> MGKIIGIDLGTTNSCVAIMDGTTPRVLENAEGDRTTPSIIAYTQDGETLVGQPAKRQAVTNPQNTLFAIKRLIGRRFQDEEVQRDVSIMPFKIIAADNGDAW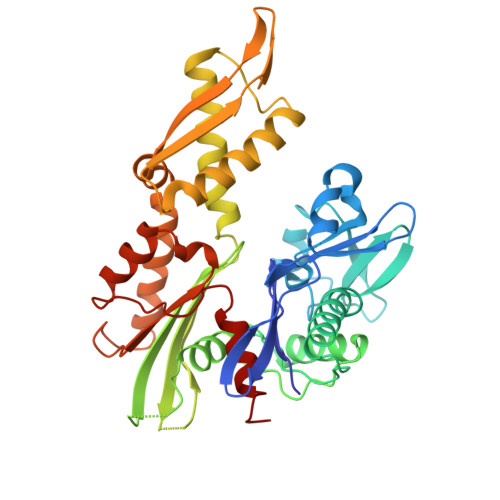VEVKGQKMAPPQISAEVLKKMKKTAEDYLGEPVTEAVITVPAYFNDAQRQATKDAGRIAGLEVKRIINEPTAAALAYGLDKGTGNRTIAVYDLGGGTFDISIIEIDEVDGEKTFEVLATNGDTHLGGEDFDSRLINYLVEEFKKDQGIDLRNDPLAMQRLKEAAEKAKIELSSAQQTDVNLPYITADATGPKHMNIKVTRAKLESLVEDLVNRSIELLKVALQDAGLSVSDIDDVILVGGQTRMPMVQKKVAEFFGKEPRKDVNPDEAVAIGAAVQGGVLT>MGSSHHHHHHSQDPENLYFQSMIPQFVIPLTNCLGQSYHFSSQPIPKGEHKKFDSEQSAKAFLDDFVPLRSSRVEELYHLLGQFPPNVPDEELTPELYAPVFAKALVNGSLYVASFPKTKKNATISSEPTPVPKQVKAKSKQNKAHTSSKTQAKNSASAKPLQTGSECHEKAGDPVSLVTGEEILTLNDVELPNGFVWSRTYRSSKASRNQGLGYGWRHAFQFELKEVTDEKHNVTSWEFISDSADEIEFEPVEHGSTSYQVYVGASCHFLNPNIRIVTLSSGDQYRFELVEDIWLLKQVRNGIFSTFQLRYSRNHRLIEVAHNKRPVLECQYDKQGRLVELLNAKTEQVLTTYIYDEQDDLVGATNDLGLTERYEYQDQHLIAKRVRPTGFTHYFEWSGEGSSAKCIRNFGDSGIYDYRFHYEGAKSSYSDSLDNEWTFIHDEQGHLLEKSSPTGRTWQWHYDHLGRKEKAVFPDNSTTQYQYNQQGQLISKLHSSGAQIQYGYDSLGKLVKTVSPDGDLEKAYYNSLGQRVWDIDALGCVTEYEYDKHGQVVKRESEDGKKSRWWWDKQQRLVAHEVDGTLLRYSYGATDLVNGIAYPDGCVAQISYDDYGRRTSIRYFNDEDKVGYSEEYAYDEFSRVAQIQTPEGVTSYQWGALAQQEAVIFPDGSHISYEYDQQRNLTKLVRSDGLAFEFWYDSEGLLSGTVGFDGLHSQFKYDSMGRIIRKDVADRTVLYSYDDAGFLQHIKAGNGKNIVENHFNYTLGGRLTLASNRHQTLQYQYSSFGHLTKRIQGQFEIGEEFNRVGQRVSQTLPDKTSFNFSYDTNGRLSEIRFSDDSLPKIEFQYDVMGRLSVTETESFRESKLYDGVGRLVEQQWSGREKKYIYNAQNRISSILDNTAGATHYQYDTLGYVTKVSEAGSTSTFESDSFGNPALADSKVMSDRIEAYAGVRYKYDQQGNQVKREGDGTVQKRVFDALSQL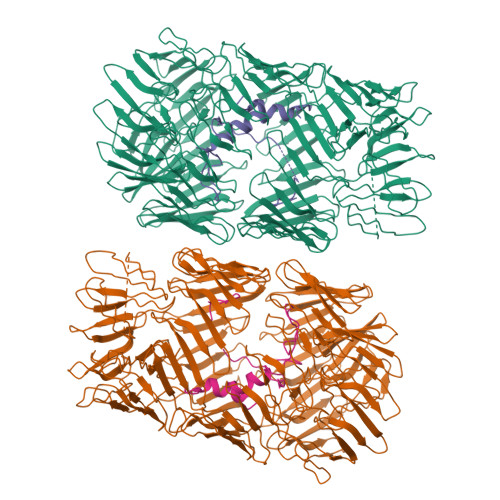VEVHGDSSISHYEYDALGRRTKKITQNGITEFLWEGERLLGERTADGFRWYLYQPETYIPLAVLENGSIYLYECDQVGKPERLKDSAGNIVWSASYDVHGFASIDVEEVRNPLRFQGQYFDQETNLHYNLARYYDPKLGRFIQQDPISIAGGINHYQYAVNPIQWIDPTGF[2x];>[2x]LCEEGLKRLQQMLAEYQAQSDVPQEVCDQILEAAKESSVGEDGVRSQVKIRKPNGKNNIRYEYDLDHIDCKKNEITFYRHINYSDGSKRKIQYTVGIEGFVDIYDFVNVQKCDAQVYDTKTSKTVGGRKIINSEFAGKTVTTKGGDVRFDSDGFPDFTPYSKKTVRVIGLTGDMANDVPLAMARAKITKYDKSKYVWHHHQDGKTMMLIPKSVHSVRNGGVAATGGRSVIQHNLLNPNNKLNYSSPEELV> MVL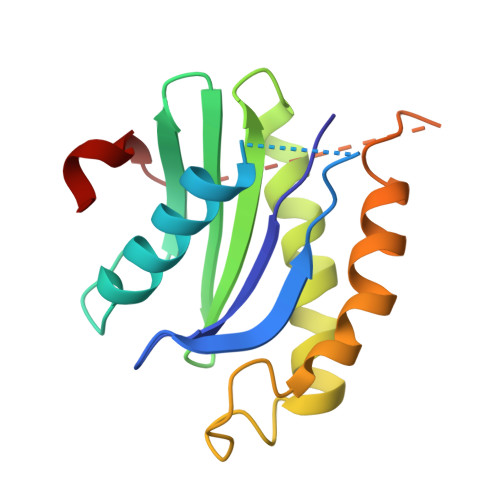LTMIARVADGLPLAASMQEDEQSGRDLQQYQSQAKQLFRKLNEQSPTRCTLEAGAMTFHYIIEQGVCYLVLCEAAFPKKLAFAYLEDLHSEFDEQHGKKVPTVSRPYSFIEFDTFIQKTKKLYIDSRARRNLGSINTELQDVQRIMVANIEEVL> XKHH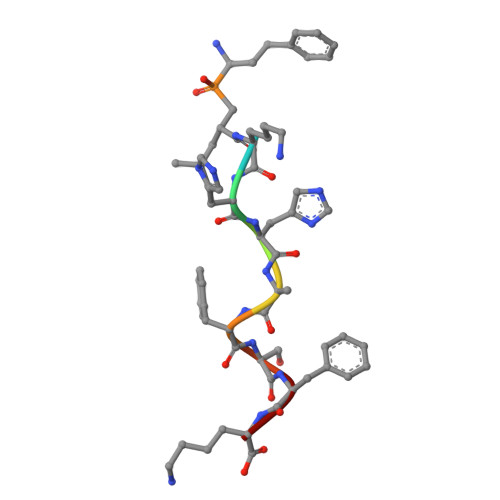AFSFK>MQLRSVIAADHPALFALWSRTPGIRLRAEDAYPFFLAYLQRNPGLSLLVETEGEVIACLMAGHDGRRGYLQHLVVDPGYRGLGLARRMLDEVLARLAREGIGKSHVFVLDAAEEAQAFWRAQSD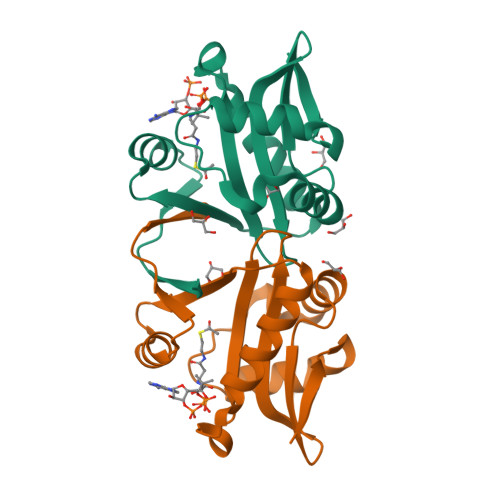WERRKDIQVFSTR[7x]>[4x]MAMKISVSKNDLENALRYLQAFLDKKDASSIASHIHLEVIKEKLFLKASDSDIGLKSYIFTQSSDKEGVGTINGKKFLDIISCLKDSNIILETKDDSLAIKQNKSSFKLPMFD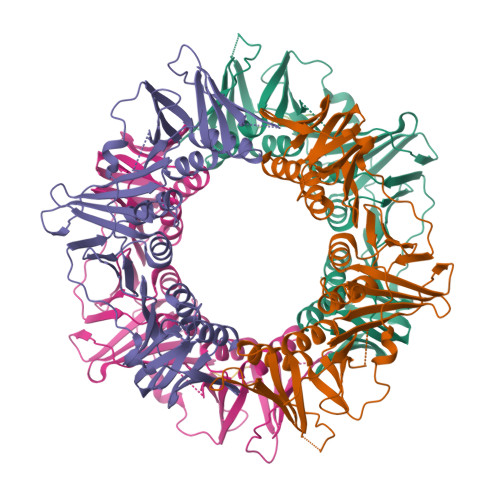ADEFPEFPVIDPKVSIEVNAPFLVDAFKKIAPVIEQTSHKRELAGILMQFDQKHQTLSVVGTDTKRLSYTQLEKISIHSTEEDISCILPKRALLEILKLFYENFSFKSDGMLAVIENEMHTFFTKLIDGNYPDYQKILPKEYISSFTLGKEEFKESIKLCSSLSSTIKLTLEKNNALFESLDSEHSETAKTSVEIEKGLDIEKAFHLGVNAKFFLEALNALGTTQFVLRCNEPSSPFLIQESLDEKQSHLNAKISTLMMPITLELHHHHHH;>QEFIRSLF[2x]> AAAKTPSSEESGLPKLPVPPLQQTLATYLQCMRHLVSEEQFRKSQAIVQQFGAPGGLGETLQQKLLERQEKTANWVSEYWLNDMYLNNRLALPVNSSPAVIFARQHFPGTDDQLRFAASLISGVLSYKALLDSHSIPTDCAKGQLSGQPLCMKQYYGLFSSYRLPGHTQDTLVAQNSSIMPEPEHVIVACCNQFFVLDVVINFRRLSEGDLFTQLRKIVKMASNAAARLPPIGLLTSDGRSEWAEARTVLVKDSTNRDSLDMIERCICLVCLDAPGGVELSDTHRALQLLHGGGYSKNGANRWYDKSLQFVVGRDGTCGVVCEHSPFDGIVLVQCTEHLLKHMTQPELVRSPMVPLPAPRRLRWKCSPEIQGHLASSAEKLQRIVKNLDFIVYKFDNYGKTFIKKQKCSPDAFIQVALQLAFYRLHRRLVPTYESASIRRFQEGRVDNIRSATPEALAFVRAVTDHKAA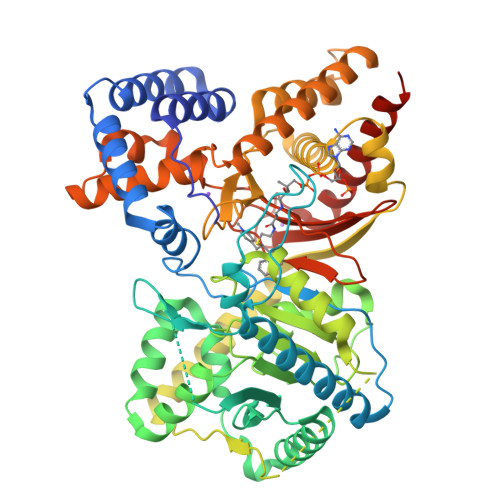VPASEKLLLLKDAIRAQTAYTVMAITGMAIDNHLLALRELARAMCAALPEMFMDETYLMSNRFVLSTSQVPTTTEMFCCYGPVVPNGYGACYNPQPETILFCISSFHSCAATSSSKFAKAVEESLIDMRDLCSLLPPTESKPL> AATQQEIMKNMWDPFQSMRAVTGLMELTSGQCTQLSKDAAAILAGVKESHDSISVDKNYKVLNDEV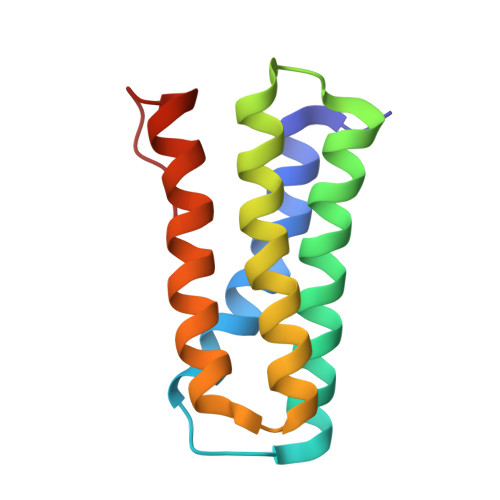AYHAANIDAAAKANDLEEVQVQFRRMTIACRNCHKIYKTEQRLVP>MRYIVALTGGIGSGKSTVANAFADLGINVIDADIIARQVVEPGAPALHAIADHFGANMIAADGTLQRRALRERIFANPEEKNWLNALLHPLIQQETQHQIQQATSPYVLWVVPLLVENSLYKKANRVLVVDVSPETQLKRTMQRDDVTREHVEQILAAQATREARLAVADDVIDNNGAPDAIASDVARLHAHYLQLASQFVSQEKPELHH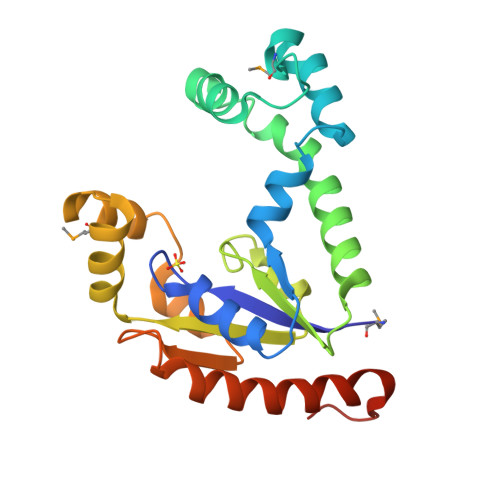HHHH[3x]>MNSLLRLPALKRGVFTMSKRGLATTVSPKTRTSNLKNGLTIASESNPLVQTATVGVWIDAGSRNENAYNNGTAHFFEHLAFKGTDKRSQHQLELDIENMGGHLNAYTSRESTVYYAKSFKDDVPKSVEILADILQHSKLAESAIDREREVITRELEEVNKQYEEVVFDHLHATAFMNQPLGRTILGPRENIQTITNTELRKFITENYTADRMVLVGAGAVDHDALVELAEKYFSHLPSSQSPVPLGTPRSSGEDANQNPIPNFVGSEVRLRDDTMPVAHIAIAVEGVSWTSEDYYTALVAQAIIGNYDRAVGTSRHQGSRLSNIVSENNLANSFQSFSTSYSDTGLWGIYLTSENTTQIDDLVHFTLKEWNRLSTSVSNLQVERAKSQLKAGLLLSLDGTTYVAEDIGRQLTTLGRRVTPAEVEAKLEAVTEHDVRAWAQKTLYDKDIALVGLGPIEGLYDYNRIRNDMSMMRW[2x];>[2x]MTRGVPRLAVAARHFSTAEAAGVKVAAQDGQSPISDLSVVLRGGSRYATVPGVSHILEKFAFQNTVPKSALRFVRELELFGGKLYTHTTREHIVLRTQFLKQDLPYFVDAFANVLKETKFQQFELTERVAPVAELDLLKRESDPAFTALEAAHEVAFRTGLGNSVYAQGYSPVTLEDVKEFARQVYAKQNVAVVGNNVVPADLQQLVGTAFADLQEGSKVTQAGTTTLHGGEARVRTSTGNALTIALPIAEPKPVYHALASFLGGPASMPWSVGASPLAQATVGTHTSVKATYHNYGDAGLFAITIKGDSPAEISQVAHKAVQALKDTGAEVTEEQAARAYAKSKFAAAEAFENPDSSASVIGMELLSGVSRIAPENVQKFTPAELSEAAAQLSASAKPVVAAVGQVHALPFADELF;>MALRKKNSLLNMANSYVLDSPQPSNLNYFWNFGSLLALCLVIQLATGITLAMHYTSHASLAFDSVEHIMRDVNFGWFIRYAHANTASFFFICIYAHMGRNIYYGSYKTPRVLPWSIGVIIFLLLIITAFMGYVLVFGQMSLWGATVICNLVSAIPWLGEDIVHFLWGGFSVGNPTLQRFFALHYLMPFVLAVFALLHLIALHTAGSSNPLGITSNVDKLSMHPYYSFKDLITVFAFLLMFTLFVFFSPDKLGHPDNYIPANPMVTPASIVPEWYLLPFYAILRAIPDKLGGVIAMVAAILILLILPIVDRSIIRGNAFKPISKLLFGFFICNFLLLGVLGQVHIEPPFIVLGQICTIFYFSYFLILLPMVSTIENIFFYIGSLRK[2x];>[2x]MRRRRIGVWPENRRVSRLWVSLSPRSCVTCPVPTNQNPPINNHHTPILTQMFKAIPLRQALLGISSAVCAGATTTYYYTTKAEAMTAAEHGLHPAEYPWPQNGMLSTFDHASLRRGYQVYKEVCAACHSLDRIAWRNLVGVTHTTDEAKAFAEELEYDDEPDDEGNPRKRPGKLADYIPGPYPNEQAARAANQGALPPDLSLIAKARHGGADYIFALLTGYPDEPPAGVVLAPGMNYNPYFPGGGIGMARTLFDGVVEYEDGTPATTSQMAKDVAAFLTWAAEPEHDERKKLGLKAIIVISAMLGLSVYIKKFKWSPIKNRKFIYNPPKN;>MSLLRTAAQAVKAPKAYTPLVAAKAFAQTRSVSSQPIGGKSTYKIPDFTPYLKKDRNTDANRLFSYFMIGSFGMLSAAGAKATVQDFLSNMSASADVLAMAKVEVKLGAIPLGKNVIIKWRGKPIFIRHRTSEEIEEANEVNVATLRDPQTDDERVQKPEWLVMIGVCTHLGCVPIGEAGDFGGWFCPCHGSHYDISGRIRRGPAPLNLEIPEYDFADAETLVIG[2x];>MSYFLTLASEVAESLLPTVAFASEEEKEQDEPVEVESDDDESEEKEDDDEEEDEDDDDDDDDDEVPDPAIALHEAAAEGPCHDFKHHFDECVERVTKAQEAEDYDHAEYKEDCVEEFFHLQHCINDNTADKLFRVLK[2x];>[2x]MASITSVVKTSELILKSPLLSKIVVPLAKTYVKFSGYRQLGFKMNDLIIEETPNMQLALRRLPPTESYDRVYRLIRATQFSLSHKLATGNDITKPEEDDHYLIPYILDVEAEAFEKDALDNLEVVKRK;>MGGNGHYMGWWGHMGSPPQKGIAGYTISPFAARPFAGVVHAAIFNTFRRTKNQALFVILPVSFFYYVWTQASEKNEWLYTKAGRHELAKALAE[2x];>[2x]MAWATTFYNVFVKRNSAFVATILASAFVFDMTFETAIDNFWDRINAGKQWKDIRHKYIEAAGDDDEDD;>MICGEGDYVKKPSYKIVPHFLGFNIPTVSKWIPIFGIWGAAAGIGALFLIEGVPRTRQDILSKIPIIGEHWIREIPASDNPF[2x]

The cytochrome bc 1 complex, also known as respiratory complex III (CIII), in the electron-transfer chain of the inner mitochondrial membrane is a homodimer (CIII2) of two biochemically identical protomers. CIII2 catalyses the transfer of electrons from the lipophilic two-electron donor ubiquinol (QH2) to the water-soluble, one-electron acceptor protein cytochrome c, contributing to an electrochemical proton gradient across the membrane. Electron transfer within the complex occurs through the prosthetic groups of the three catalytic core subunits: heme b L and heme b H of cytochrome b (cyt b), heme c 1 of cytochrome c 1 (cyt c 1) and the [2Fe–2S] cluster of the iron–sulfur protein (ISP), often called the Rieske protein after its discoverer. The Rieske domain is tethered to the complex by one transmembrane helix and a connecting flexible linker that acts as a hinge.

In intermediate positions, the tip of the Rieske domain is close to the ef-loop of cyt b. Map density for the Rieske domain was less good at positions in which the cluster-bearing tip did not interact closely with either cyt b or cyt c 1. In maps of fully reduced or oxidized samples this area of cyt b was well-resolved irrespective of the position of the Rieske domain. The addition of antimycin A reduced the resolution of these regions, whereas both the cd 1-helix and the ef-loop were well-resolved in the intermediate positions of CIII2 oxidized with ferricyanide or reduced with ascorbate or DQH2. Despite the closer interaction of the Rieske domain with cyt b, no shift in the equilibrium of positions in ascorbate-reduced samples was observed.> TKQTARKSTG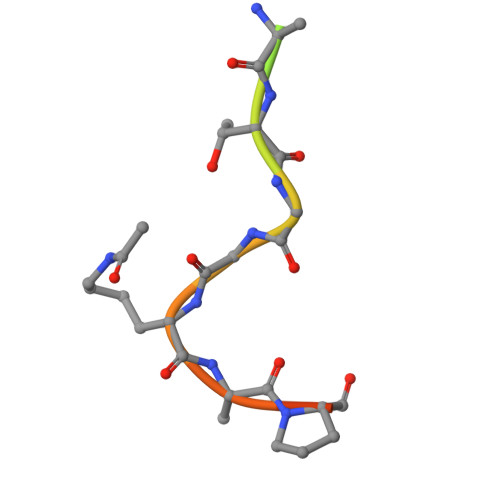GKAPRKQ> SETEL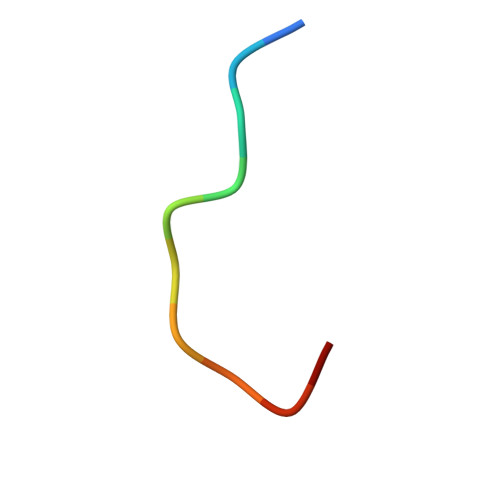DLALGL5-bromo-7-{5-[(3-{[(4-tert-butylphenyl)carbamoyl]amino}propyl)amino]-5-deoxy-beta-D-ribofuranosyl}-7H-pyrrolo[2,3-d]pyrimidin-4-amine 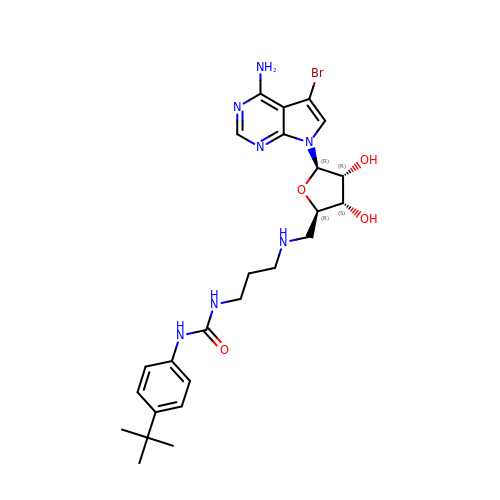| C25 H34 Br N7 O4 | RFVBTQBCRYTKHX-ZDXOVATRSA-N Factor XI (FXI) has an important role in thrombin generation in the amplification phase of the coagulation process. Inhibition of activated FXI (FXIa) should decrease thrombin generation in the amplification phase, but not in the initiation phase, and thus yield an antithrombotic and profibrinolytic effect with minimal risk of bleeding (see reviews). To improve crystallisability, the quadruple mutant (Ser75Ala, Lys78Ala, Thr97Ala and Cys123Ser), first reported by Jin et al., was generated. The mutated residues in this construct (FXIa CD) are located at least 16 Å from the catalytic residue Ser195 and the alterations are therefore not anticipated to impact ligand binding in the active site.

In parallel with the fragment hit identification work, compounds 9–11 from patent applications from Bristol Myers Squibb were synthesized and characterized. The compounds are potent FXIa and plasma prekallikrein inhibitors and selective against e.g. thrombin and FXa as seen in Fig. 6. The crystal structures of 9–11 in complex with FXIa CD were not available in the public domain and were therefore solved by X-ray crystallography. Given our aim to target the prime side, it was exciting to note the S1-S1’-S2’ binding mode for all three compounds, as shown for compound 9 in Fig. 7. None of the designed linked compounds, 20–24, reached as high potency as compound 10. However, compound 20 with an IC50 of 330 nM, suggests feasibility of including reverse amides in expanded structures. The crystal structures of compounds 9–11 in complex with FXIa CD gave a clear handle on directed expansion of fragments towards the prime side and allowed linking exercises.

> IVGGTASVRGEWPWQVTLHTTSPTQRHLCGGSIIGNQWILTAAHCFYGVESPKILRVYSGILNQAEIAEDTSFFGVQEIIIHDQYKMAESGYDIALLKLETTVNYADSQRPISLPSKGERNVIYTDCWVTGWGYRKLRDKIQNTLQKAKIPLVTNEECQKRYRGHKITHKMICAGYREGGKDACKGDSGGPLSCKHNEVWHLVGITSWGEGCAQRERPGVYTNVVEYVDWILEKTQAV> MADYKDDDDKSGPDEVDASGRMAVLRQLALLLWKNYTLQKRKVLVT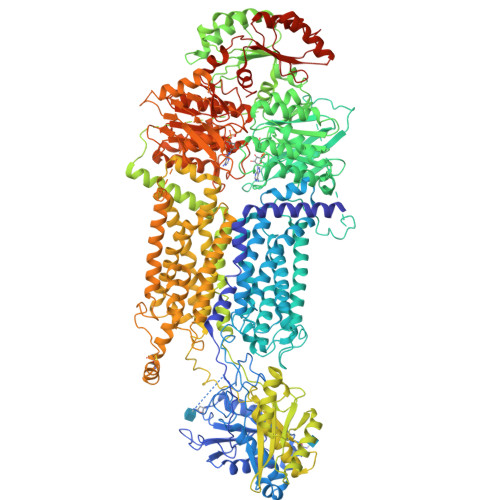VLELFLPLLFSGILIWLRLKIQSENVPNATIYPGQSIQELPLFFTFPPPGDTWELAYIPSHSDAAKTVTETVRRALVINMRVRGFPSEKDFEDYIRYDNCSSSVLAAVVFEHPFNHSKEPLPLAVKYHLRFSYTRRNYMWTQTGSFFLKETEGWHTTSLFPLFPNPGPREPTSPDGGEPGYIREGFLAVQHAVDRAIMEYHADAATRQLFQRLTVTIKRFPYPPFIADPFLVAIQYQLPLLLLLSFTYTALTIARAVVQEKERRLKEYMRMMGLSSWLHWSAWFLLFFLFLLIAASFMTLLFCVKVKPNVAVLSRSDPSLVLAFLLCFAISTISFSFMVSTFFSKANMAAAFGGFLYFFTYIPYFFVAPRYNWMTLSQKLCSCLLSNVAMAMGAQLIGKFEAKGMGIQWRDLLSPVNVDDDFCFGQVLGMLLLDSVLYGLVTWYMEAVFPGQFGVPQPWYFFIMPSYWCGKPRAVAGKEEEDSDPEKALRNEYFEAEPEDLVAGIKIKHLSKVFRVGNKDRAAVRDLNLNLYEGQITVLLGHNGAGKTTTLSMLTGLFPPTSGRAYISGYEISQDMVQIRKSLGLCPQHDILFDNLTVAEHLYFYAQLKGLSRQKCPEEVKQMLHIIGLEDKWNSRSRFLSGGMRRKLSIGIALIAGSKVLILDQPTSGMDAISRRAIWDLLQRQKSDRTIVLTTHFMDEADLLGDRIAIMAKGELQCCGSSLFLKQKYGAGYHMTLVKEPHCNPEDISQLVHHHVPNATLESSAGAELSFILPRESTHRFEGLFAKLEKKQKELGIASFGASITTMEEVFLRVGKLVDSSMDIQAIQLPALQYQHERRASDWAVDSNLCGAMDPSDGIGALIEEERTAVKLNTGLALHCQQFWAMFLKKAAYSWREWKMVAAQVLVPLTCVTLALLAINYSSELFDDPMLRLTLGEYGRTVVPFSVPGTSQLGQQLSEHLKDALQAEGQEPREVLGDLEEFLIFRASVEGGGFNERCLVAASFRDVGERTVVNALFNNQAYHSPATALAVVDNLLFKLLCGPHASIVVSNFPQPRSALQAAKDQFNEGRKGFDIALNLLFAMAFLASTFSILAVSERAVQAKHVQFVSGVHVASFWLSALLWDLISFLIPSLLLLVVFKAFDVRAFTRDGHMADTLLLLLLYGWAIIPLMYLMNFFFLGAATAYTRLTIFNILSGIATFLMVTIMRIPAVKLEELSKTLDHVFLVLPNHCLGMAVSSFYENYETRRYCTSSEVAAHYCKKYNIQYQENFYAWSAPGVGRFVASMAASGCAYLILLFLIETNLLQRLRGILCALRRRRTLTELYTRMPVLPEDQDVADERTRILAPSPDSLLHTPLIIKELSKVYEQRVPLLAVDRLSLAVQKGECFGLLGFNGAGKTTTFKMLTGEESLTSGDAFVGGHRISSDVGKVRQRIGYCPQFDALLDHMTGREMLVMYARLRGIPERHIGACVENTLRGLLLEPHANKLVRTYSGGNKRKLSTGIALIGEPAVIFLDQPSTGMDPVARRLLWDTVARARESGKAIIITSHSMEECEALCTRLAIMVQGQFKCLGSPQHLKSKFGSGYSLRAKVQSEGQQEALEEFKAFVDLTFPGSVLEDEHQGMVHYHLPGRDLSWAKVFGILEKAKEKYGVDDYSVSQISLEQVFLSFAHLQPPTAEEGRLEGSDEVDAVEGSHHHHHHHHHH> ASRYLTDMTLEEMSRDWFMLMPKQKVAGSLCIRMDQAIMDKNIILKA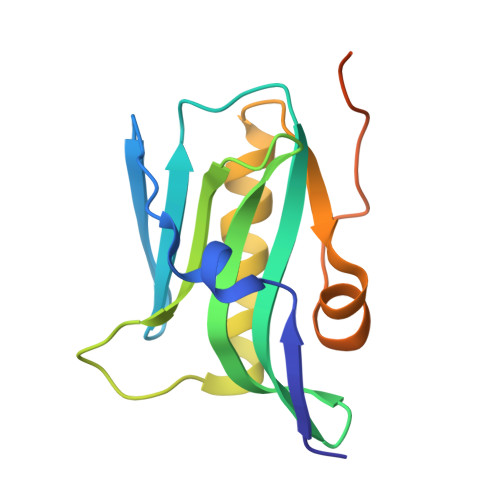NFSVIFDRLETLILLRAFTEEGAIVGEISPLPSLPGHTDEDVKNAVGVLIGGLEANDNTVRVSETLQRFAWRSSNENGRPPLPPKQKRKMARTIKSEV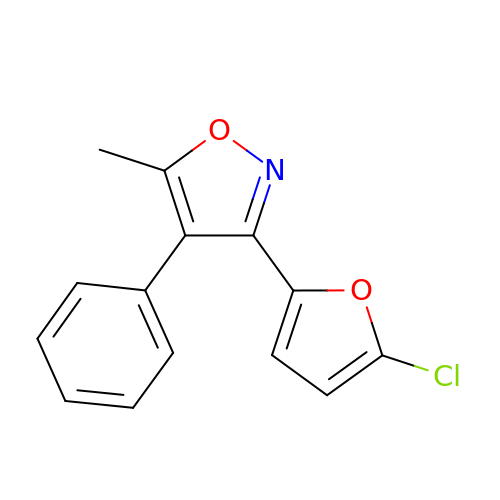3-(5-chlorofuran-2-yl)-5-methyl-4-phenyl-1,2-oxazole | C14 H10 Cl N O2 | IPAVFMUBTIUYBW-UHFFFAOYSA-N> MMVISEKVRKALNDQLNREIYSSYLYLSMATYFDAEGFKGFAHWMKKQAQEELTHAMK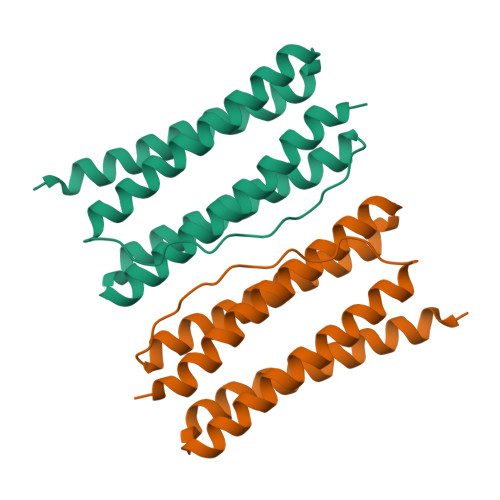FYEYIYERGGRVELEAIEKPPSNWNGIKDAFEAALKHEEFVTQSIYNILELAFEEKDHATVSFLKWFVDEQVEEEDQVREILDLLEKANG5-methyl-6-quinolin-5-yl-3~{H}-quinazolin-4-one | C18 H13 N3 O | 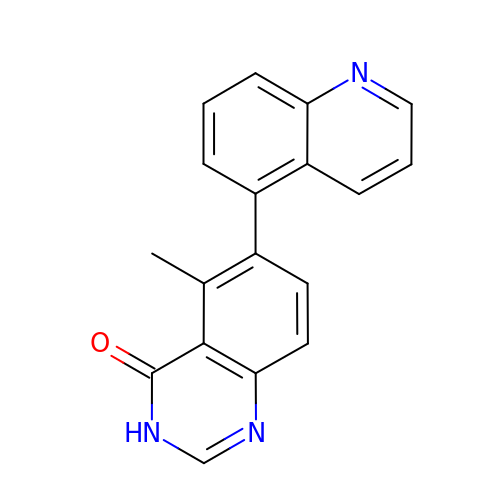UUGUFBFLQOTDIV-UHFFFAOYSA-N The CG11501 gene encodes a small cysteine-rich protein that we named Diedel. Diedel is 115 amino acids long and contains 10 cysteines. The CG11501 gene was identified as a negative regulator of the JAK/STAT signaling pathway in this study, although its precise molecular function is still unknown. The overall structure shows a relatively elongated shape with approximate dimensions of 60×40×40 Å3, which can be divided into two sub-domains referred as SD1 and SD2.

Form A crystals belonged to the orthorhombic space group P212121, with unit-cell parameters a = 29.83 Å, b = 44.30 Å and c = 58.54 Å. The structure was solved by the SIRAS method using an iodo derivative and was refined to an R factor of 12.9% and an R-free factor of 15.1% to 1.15 Å resolution. The final model for form A includes the entire expressed protein from residue 25 to 115, the 24 first residues being the signal peptide that is cleaved upon exportation, two extra residues (116 and 117) being cloning artifacts, one thiocyanate molecule, one ethylene glycol molecule and 144 water molecules. The SD1 sub-domain is made of two segments 29–59 and 90–117, and is composed of a four stranded anti parallel β-sheet (30–35, 48–49, 55–59, 109–113), one α-helix (92–99) and two 310 turns (43–46 and 100–103). The SD2 sub-domain is formed by the first four N-terminal residues (25–28) and by a long loop (residues 60 to 89) connecting the strand β3 and the α-helix of the sub-domain SD1. This domain is highly reticulated with four disulfide bridges; two of them tether the loop 60–89 to the N-terminal residues. The main structural difference is located in the loop 51–54 with a distance between the Cα atoms of more than 5 Å for the residue 53. The change in the main chain trace is the result of a difference of peptidyl isomerization for the proline 52. Indeed this residue is in cis conformation in form A and in trans conformation in form B. Nevertheless positioning the structure found in form A in the crystal packing of form B leads to several clashes (distance below 1.5 Å) between Pro52 and Gly85 of a symmetry related molecule. This is also the case, but in a lesser extend, when putting form B structure in form A crystal packing with few short contacts between Y51 and I48 of a symmetry related molecule.

> ECCTSRELVEFKMDRGDCEAVRAIENYPNGCEVTICADGVAQLGAYCGQGPCNIFGCNCDGGCLSGDWSQEFVRRNQQYGIQIIKVTRLPFWRPL> MINQVYQLVAPRQFEVTYNNVDIYSDYVIVRPLYMSICAADQRYYTGSRDENVLSQKLPMSLIHEGVGEVVFDSKGVFNKGTKVVMVPNTPTEKDDVIAENYLKSSYFRSSGHDGFMQDFVLLNHDR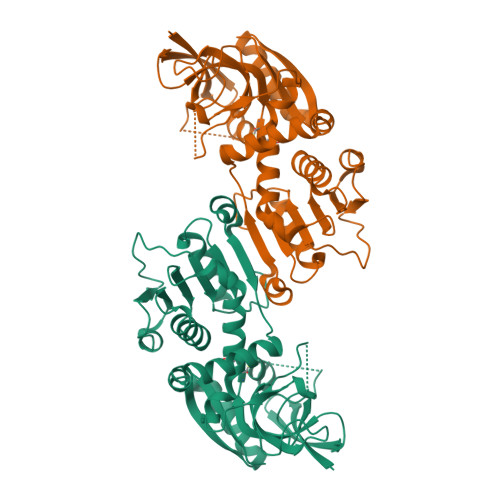AVPLPDDIDLSIISYTELVTVSLHAIRRFEKKSISNKNTFGIWGDGNLGYITAILLRKLYPESKIYVFGKTDYKLSHFSFVDDVFFINKIPEGLTFDHAFECVGGRGSQSAINQMIDYISPEGSIALLGVSEFPVEVNTRLVLEKGLTLIGSSRSGSKDFQDVVDLYIQYPDIVDKLALLKGQEFEIATINDLTEAFEADLSTSWGKTVLKWIM> GPVEESVDRAVARVADTISSRPTNSESIPALTAAETGHTSQVVPSDTMQTRHVKNYHSRSESSIENFLCRSACVYYATYTNNSKKGFAEWVINTRQVAQLRRKLELFTYLRFDLELTFVITSAQQPSTASSVDAPVQTHQIMYVPPGGPVPTKVKDYAWQTSTNPSVFWTEGNAPPRMSIPFISIGNAYSCFYDGWTQFSRNGVYGINTLNNMGTLYMRHVNEAGQGPIKSTVRIYFKPKHVKAWVPRPPRLCQYEKQKNVNFSPIGVTTSRTDIITT;> SPSAEECGYSDRVRSITLGNSTITTQECANVVVGYGVWPEYLKDNEATAEDQPTQPDVATCRFYTLESVQWMKNSAGWWWKLPDALSQMGLFGQNMQYHYLGRTGYTIHVQCNASKFHQGCLLVVCVPEAEMGCSNLNNTPEFSELSGGDSARMFTDTQVGESNAKKVQTAVWNAGMGVGVGNLTIFPHQWINLRTNNSATLVMPYINSVPMDNMFRHNNLTLMIIPFVPLNYSEGSSPYVPITVTIAPMCAEYNGLRLASNQ;> GLPVMTTPGSTQFLTSDDFQSPSAMPQFDVTPEMQIPGRVNN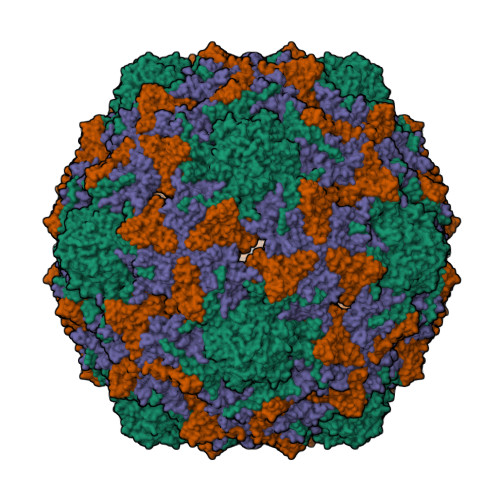LMEIAEVDSVVPVNNTEDNVSSLKAYQIPVQSNSDNGKQVFGFPLQPGANNVLNRTLLGEILNYYTHWSGSIKLTFMFCGSAMATGKFLLAYSPPGAGVPKNRKDAMLGTHVIWDVGLQSSCVLCVPWISQTHYRYVVEDEYTAAGYVTCWYQTNIVVPADVQSSCDILCFVSACNDFSVRMLKDTPFIRQDTFYQ>GTNIRVAIVGYGNLGRSVEKLIAKQPDMDLVGIFSRRATLDTKTPVFDVADVDKHADDVDVLFLCMGSATDIPEQAPKFAQFACTVDTYDNHRDIPRHRQVMNEAATAAGNVALVSTGWDPGMFSINRVYAAAVLAEHQQHTFWGPGLSLGHSGALRRIPGVQKAVQYILPSEDALEKARRGEAGDLTGKQTHKMQCFVVADAADHERIENDIRTMPDYFVGYEVEVNFIDEATFDSEHTGMPNGGHVITTGDTGGFNHTVEYILKLDRNPDFTASSQIAFGRAAHRMKQQGQSGAFTVLEV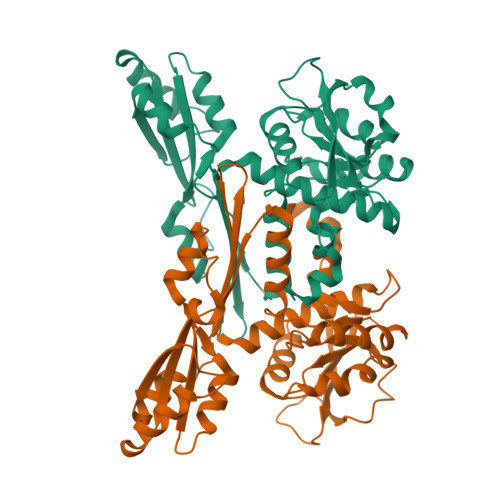APYLLSPENLDDLIARDV[2x]>[3x]QGMSKIFGIVNITTDSFSDGGLYLDTDKAIEHALHLVEDGADVIDLGAASSNPDTTEVGVVEEIKRLKPVIKALKEKGISISVDTFKPEVQSFCIEQKVDFINDIQGFPYPEIYSGLAKSDCKLVLMHSVQRIGAATKVETNPEEVFTSMMEFFKERIAALVEAGVKRERIILDPGMGFFLGSNPETSILVLKRFPEIQEAFNLQVMIAVSRKSFLGKITGTDVKSRLAPTLAAEMYAYKKGADYLRTHDVKSLSDALKISKALG

The sulfonamides (sulfas) are the oldest class of antibacterial drugs and inhibit the bacterial dihydropteroate synthase (DHPS, encoded by folP), through chemical mimicry of its co-substrate p-aminobenzoic acid (pABA). Resistance to sulfa drugs is mediated either by mutations in folP or acquisition of sul genes, which code for sulfa-insensitive, divergent DHPS enzymes. DHPS catalyzes the condensation of para-aminobenzoic acid (pABA) and 6-hydroxymethyl-7,8-dihydropterin pyrophosphate (DHPP), producing 7,8-dihydropteroic acid (7,8-DHP); this compound is further transformed, ultimately leading to tetrahydrofolate, an essential precursor for DNA and RNA synthesis. All three Sul enzymes adopted the (ɑ/β)8 TIM barrel fold also shared by DHPS.

We determined the crystal structure of Sul1 in a ligand-bound state, and the Sul2 and Sul3 enzymes in both apo and ligand-bound forms to resolutions between 1.74 to 2.8 Å. Comparison of Sul apo and ligand-bound structures revealed conformational changes in these three loops triggered by ligand binding. We noticed that the Phe residue that is conserved across Sul enzymes (Phe178 in Sul1, Phe179 in Sul2 and Phe177 in Sul3) and localized to the active site adopted different rotamer conformations depending on ligand binding.The underlying channels, termed volume-regulated anion channels (VRACs) have variable selectivity and conductance between cells, but are similarly activated by osmotic stimuli and blocked by small molecule anionic inhibitors including DCPIB (4-[(2-Butyl-6,7-dichloro-2-cyclopentyl-2,3-dihydro-1-oxo-1H-inden-5-yl)oxy]butanoic acid). LRRC8A forms a 565 kDa, homohexameric channel with each monomer consisting of (from extracellular to intracellular side) an extracellular cap, four transmembrane spanning helices TM1-4, a linker region, and a LRR domain. Here, we report structures of the homohexameric LRRC8A channel embedded in lipid nanodiscs in the presence and absence of the inhibitor DCPIB determined by cryo-electron microscopy. The N-terminal arginine residue of this helix (R103) projects in towards the conduction axis to form the highly electropositive selectivity filter of the anion-selective channel.

Focused classification on the linker region and lower portion of the TMs resolved a constricted and an expanded state of LRRC8A. Alignment of the two structures by the extracellular cap shows that the differences are confined to the cytoplasmic halves of the TMs, linker regions, and LRRs. The differences can be approximated as a rigid body displacement of the lower portion of the channel about hinges approximately half way through each transmembrane helix. This generates displacements of ~2–4 Å in the cytoplasmic ends of the transmembrane helices, the linkers, and at the cytoplasmic connection between the linkers and LRRs. As a consequence of these conformational changes, the channel cavity is markedly larger in the expanded state: it dilates approximately 4 Å including at the first resolved N-terminal residue (Pro15). The conformational changes we observe show how expansion of cytoplasmic ionic-strength sensing regions can be coupled to expansion of N-terminal gating regions and the channel pore. Still, it is tempting to speculate based on structural considerations that the expanded state represents an intermediate on the path to a fully conductive channel. The 4 Å increase in channel cavity diameter at the position of the unresolved N-terminus represents a significant expansion, comparable in size to the selectivity filter opening and approaching the diameter of a solvated chloride ion. Still, we cannot determine whether these changes are sufficient to fully open the channel since the N-terminal 14 amino acids that project into the channel cavity are unresolved. Masking out the LRRs and applying six-fold (C6) symmetry resulted in the highest resolution reconstructions: 3.21 Å resolution for the constricted and 3.32 Å resolution for the expanded class, respectively.

>[6x]MIPVTELRYFADTQPAYRILKPWWDVFTDYISIVMLMIAVFGGTLQVTQDKMICLPCKWVTKDSCNDSFRGWAASSPEPTYPNSTVLPTPDTGPTGIKYDLDRHQYNYVDAVCYENRLHWFAKYFPYLVLLHTLIFLACSNFWFKFPRTSSKLEHFVSILLKCFDSPWTTRALSETVVEESDPKPAFSKMNGSMDKKSSTVSEDVEATVPMLQRTKSRIEQGIVDRSETGVLDKKEGEQAKALFEKVKKFRTHVEEGDIVYRLYMRQTIIKVIKFALIICYTVYYVHNIKFDVDCTVDIESLTGYRTYRCAHPLATLFKILASFYISLVIFYGLICMYTLWWMLRRSLKKYSFESIREESSYSDIPDVKNDFAFMLHLIDQYDPLYSKRFAVFLSEVSENKLRQLNLNNEWTLDKLRQRLTKNAQDKLELHLFMLSGIPDTVFDLVELEVLKLELIPDVTIPPSIAQLTGLKELWLYHTAAKIEAPALAFLRENLRALHIKFTDIKEIPLWIYSLKTLEELHLTGNLSAENNRYIVIDGLRELKRLKVLRLKSNLSKLPQVVTDVGVHLQKLSINNEGTKLIVLNSLKKMVNLTELELIRCDLERIPHSIFSLHNLQEIDLKDNNLKTIEEIISFQHLHRLTCLKLWYNHIAYIPIQIGNLTNLERLYLNRNKIEKIPTQLFYCRKLRYLDLSHNNLTFLPADIGLLQNLQNLAVTANRIEALPPELFQCRKLRALHLGNNVLQSLPSRVGELTNLTQIELRGNRLECLPVELGECPLLKRSGLVVEEDLFSTLPPEVKERLWRADKEQASNSLEVLFQG> LQTLPPVQLAQ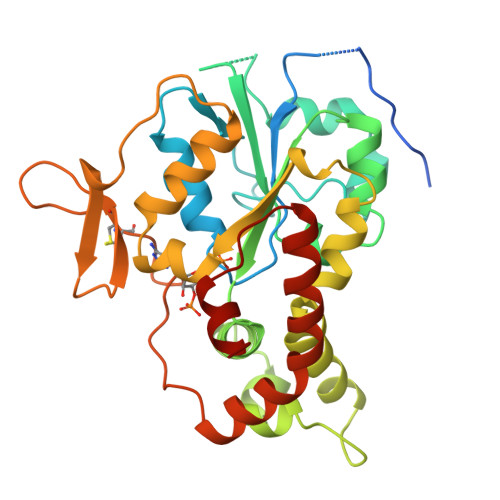KYFQIFSEEKDPLWQDPCEDKRHKDIWSKEKTCDRFPKLLIIGPQKTGTTALYLFLGMHPDLSSNYPSSETFEEIQFFNGHNYHKGIDWYMEFFPIPSNTTSDFYFEKSANYFDSEVAPRRAAALLPKAKVLTILINPADRAYSWYQHQRAHDDPVALKYTFHEVITAGSDASSKLRALQNRCLVPGWYATHIERWLSAYHANQILVLDGKLLRTEPAKVMDMVQKFLGVTNTIDYHKTLAFDPKKGFWCQLLEGGKTKCLGKSKGRKYPEMDLDSRAFLKDYYRDHNIELSKLLYKMGQTLPTWLREDLQNTR>[2x]AEKPKLHYFNARGKMESTR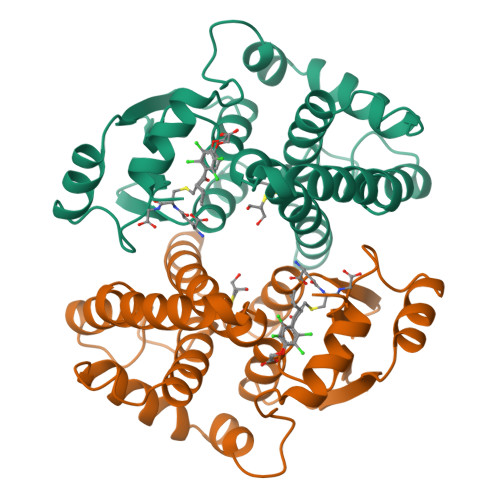WLLAAAGVEFEEKFIKSAEDLDKLRNDGYLMFQQVPMVEIDGMKLVQTRAILNYIASKYNLYGKDIKERALIDMYIEGIADLGEMILLLPVCPPEEKDAKLALIKEKIKNRYFPAFEKVLKSHGQDYLVGNKLSRADIHLVELLYYVEELDSSLISSFPLLKALKTRISNLPTVKKFLQPGSPRKPPMDEKSLEEARKIFRF> MANVWGVRLADSLSSPTIETRTRQYTLHDLCSDLDANPGREPWKPLRNQRTNNIVAVQLFRPLQGLVLDTQLYGFPGAFDDWERFMREKLRVLKYEVLRIYPISNYSNEHVNVFVANALVGAFLSNQAFYDLLPLLIINDTMIGDLLGTGASLSQFFQSHGDVLEVAAGRKYLQMENYSNDDDDPPLFAKDLSDYAKAFYSDTYEVLDRFFWTHDSSAGVLVHYDKPTNGHHYLLGTLTQMVSAPPYIINATDAMLLESCLEQFSANVRARPAQPVTRLDQCYHLRWGAQYVGEDSLTYRLGVLSLLATNGYQLARPIPRQLTNRWLSSFVSQIMSDGVNETPLWPQERYVQIAYDSPSVVDGATQYGYVRKNQLRLGMRISALQSLSDTPSPVQWLPQYTIDQAAMDEGDLMVSRLTQLPLRPDYGNIWVGDALSYYVDYNRSHRVVLSSELPQLPDTYFDGDEQYGRSLFSLARKIGDRSLVKDTAVLKHAYQAIDPNTGKEYLRSRQSVAYFGASAGHSGADQPLVIEPWIQGKISGVPPPSSVRQFGYDVARGAIVDLARPFPSGDYQFVYSDVDQVVDGHDDLSISSGLVESLLSSCMHATAPGGSFVVKINFPTRPVWHYIEQKILPNITSYMLIKPFVTNNVELFFVAFGVHQHSSLTWTSGVYFFLVDHFYRYETLSTISRQLPSFGYVDDGSSVTGIETISIENPGFSNMTQAARIGISGLCANVGNARKSIAIYESHGARVLTITSRRSPASARRKSRLRYLPLIDPRSLEVQARTILPADPVLFENVSGASPHVCLTMMYNFEVSSAVYDGDVVLDLGTGPEAKILELIPATSPVTCVDIRPTAQPSGCWNVRTTFLELDYLSDGWITGVRGDIVTCMLSLGAAAAGKSMTFDAAFQQLIKVLSKSTANVVLVQVNCPTDVVRSIKGYLEIDSTNKRYRFPKFGRDEPYSDMDALEKICRTAWPNCSITWVPLSYDLRWTRLALLESTTLSSASIRIAELMYKYMPIMRIDIHGLPMEKRGNFIVGQNCSLVIPGFNAQDVFNCYFNSALAFSTEDVNAAMIPQVSAQFDATKGEWTLDMVFSDAGIYTMQALVGSNANPVSLGSFVVDSPDVDITDAWPAQLDFTIAGTDVDITVNPYYRLMTFVRIDGQWQIANPDKFQFFSSASGTLVMNVKLDIADKYLLYYIRDVQSRDVGFYIQHPLQLLNTITLPTNEDLFLSAPDMREWAVKESGNTICILNSQGFVLPQDWDVLTDTISWSPSIPTYIVPPGDYTLTPL;>MKRIPRKTKGKSSGKGNDSTERSDDGSSQLRDKQNNKAGPATTEPGTSNREQYRARPGIASVQRATESAELPMKNNDEGTPDKKGNTRGDLVNEHSEAKDEADEATQKQAKDTDKSKAQVTYSDTGINNANELSRSGNVDNEGGSNQKPMSTRIAEATSAIVSKHPARVGLPPTASSGHGYQCHVCSAVLFSPLDLDAHVASHGLHGNMTLTSSEIQRHITEFISSWQNHPIVQVSADVENKKTAQLLHADTPRLVTWDAGLCTSFKIVPIVPAQVPQDVLAYTFFTSSYAIQSPFPEAAVSRIVVHTRWASNVDFDRDSSVIMAPPTENNIHLFKQLLNTETLSVRGANPLMFRANVLHMLLEFVLDNLYLNRHTGFSQDHTPFTEGANLRSLPGPDAEKWYSIMYPTRMGTPNVSKICNFVASCVRNRVGRFDRAQMMNGAMSEWVDVFETSDALTVSIRGRWMARLARMNINPTEIEWALTECAQGYVTVTSPYAPSVNRLMPYRISNAERQISQIIRIMNIGNNATVIQPVLQDISVLLQRISPLQIDPTIISNTMSTVSESTTQTLSPASSILGKLRPSNSDFSSFRVALAGWLYNGVVTTVIDDSSYPKDGGSVTSLENLWDFFILALALPLTTDPCAPVKAFMTLANMMVGFETIPMDNQIYTQSRRASAFSTPHTWPRCFMNIQLISPIDAPILRQWAEIIHRYWPNPSQIRYGAPNVFGSANLFTPPEVLLLPIDHQPANVTTPTLDFTNELTNWRARVCELMKNLVDNQRYQPGWTQSLVSSMRGTLDKLKLIKSMTPMYLQQLAPVELAVIAPMLPFPPFQVPYVRLDRDRVPTMVGVTRQSRDTITQPALSLSTTNTTVGVPLALDARAITVALLSGKYPPDLVTNVWYADAIYPMYADTEVFSNLQRDMITCEAVQTLVTLVAQISETQYPVDRYLDWIPSLRASAATAATFAEWVNTSMKTAFDLSDMLLEPLLSGDPRMTQLAIQYQQYNGRTFNVIPEMPGSVIADCVQLTAEVFNHEYNLFGIARGDIIIGRVQSTHLWSPLAPPPDLVFDRDTPGVHIFGRDCRISFGMNGAAPMIRDETGMMVPFEGNWIFPLALWQMNTRYFNQQFDAWIKTGELRIRIEMGAYPYMLHYYDPRQYANAWNLTSAWLEEITPTSIPSVPFMVPISSDHDISSAPAVQYIISTEYNDRSLFCTNSSSPQTIAGPDKHIPVERYNILTNPDAPPTQIQLPEVVDLYNVVTRYAYETPPITAVVMGVP[2x];>[2x]MARAAFLFKTVGFGGLQNVPINDELSSHLLRAGNSPWQLTQFLDWISLGRGLATSALVPTAGSRYYQMSCLLSGTLQIPFRPNHRWGDIRFLRLVWSAPTLDGLVVAPPQVLAQPALQAQADRVYDCDDYPFLARDPRFKHRVYQQLSAVTLLNLTGFGPISYVRVDEDMWSGDVNQLLMNYFGHTFAEIAYTLCQASANRPWEHDGTYARMTQIILSLFWLSYVGVIHQQNTYRTFYFQCNRRGDAAEVWILSCSLNHSAQIRPGNRSLFVMPTSPDWNMDVNLILSSTLTGCLCSGSQLPLIDN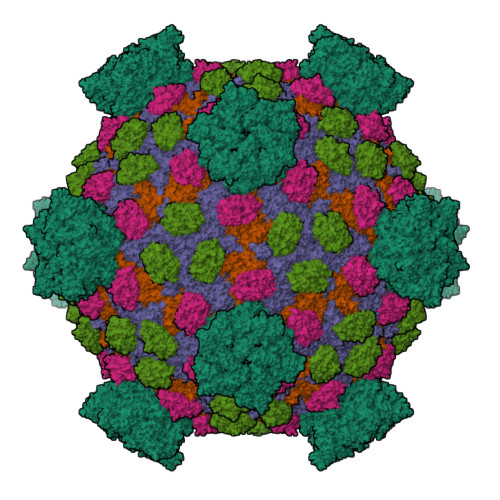NSVPAVSRNIHGWTGRAGNQLHGFQVRRMVTEFCDRLRRDGVMTQAQQNQIEALADQTQQFKRDKLEAWAREDDQYNQANPNSTMFRTKPFTNAQWGRGNTGATSAAIAALI>[2x]APDWVPPEVFDLVAE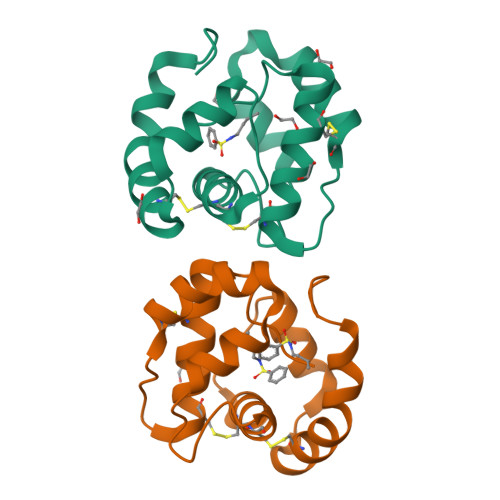DKARCMSEHGTTQAQIDDVNKGNLVNEPSITCYMYCLLEAFSLVDDEANVDEDIMLGLLPDQLQERAQSVMGKCLPTSGSDNCNKIYNLAKCVQESAPDVWFVI>[2x]GIEKIISRSMFDQMLKHRNNPACPAKGFYTYDAFIAAAKSFPSFGTTGSTDVRKREIAAFLGQTSHETTGGWPSAPDGPYAWGYCFLKERNPSSNYCAPSPRYPCAPGKS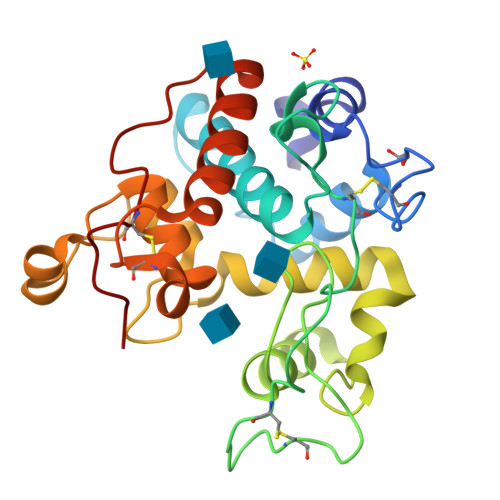YYGRGPIQLSWNYNYGPCGEALRVNLLGNPDLVATDRVISFKTALWFWMTPQAPKPSCHDVITGRWQPSAADTAAGRLPGYGVITNIINGGLECGKGPNPQVADRIGFFRRYCGILGVGTGNNLDCYNQRPFG> ASAKLPGDFGPPRGEPIHAVLTSPPLVPPPVNRTYPAKVIVELEVVEKEMQISEGVSYTFWTFGGTVPGSFIRVRQGDTVEFHLKNHPSSKMPHNIDLHGVTGPGGGAASSFTAPGHESQFTFKALNEGIYVYHCATAPVGMHIANGMYGLILVEPPEGLPKVDHEYYVMQGDFYTAGKYREKGLQPFDMEKAIDERPSYVLFNGAEGALTGDKALHAK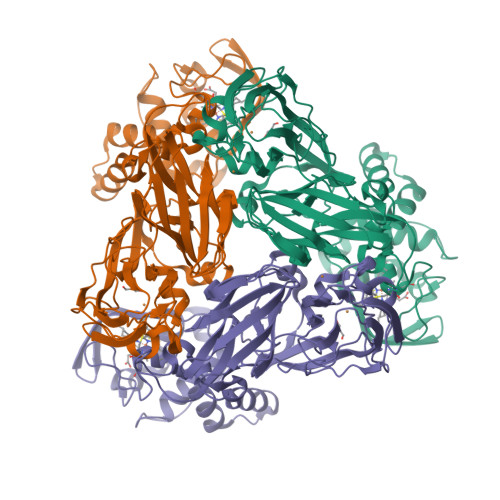VGETVRIFVGNGGPNLVSSFHVIGAIFDQVRYEGGTNVQKNVQTTLIPAGGAAVVKFTARVPGSYVLVDHSIFRAFNKGAMAILKIDGAENKLVYSGKELDSVFLGDRAAPNMSAVTKATQASVSGTLTVQDQVQAGRALFAGTCSVCHQGNGAGLPGVFPPLAKSDFLAADPKRAMNIVLHGLNGKIKVNGQEYDSVMPPMTQLNDDEVANILTYVLNSWDNPGGRVSAEDVKKVRAQPAPAKAVAEH>TQPALLRLSDHLLANYKKGVRPVRDWRKPTTVSIDVIMYAILNVDEKNQVLTTYIWYRQYWTDEFLQWTPEDFDNVTKLSIPTDSIWVPDILINEFVDVGKSPNIPYVYVHHRGEVQNYKPLQLVTACSLDIYNFPFDVQNCSLTFTSWLHTIQDINITLWRSPEEVRSDKSIFINQGEWELLEVFPQFKEFSIDISNSYAEMKFYVIIRRRPLFYAVSLLLPSIFLMVVDIVGFCLPPDSGERVSFKITLLLGYSVFLIIVSDTLPATAIGTPLIGVYFVVCMALLVISLAETIFIVRLV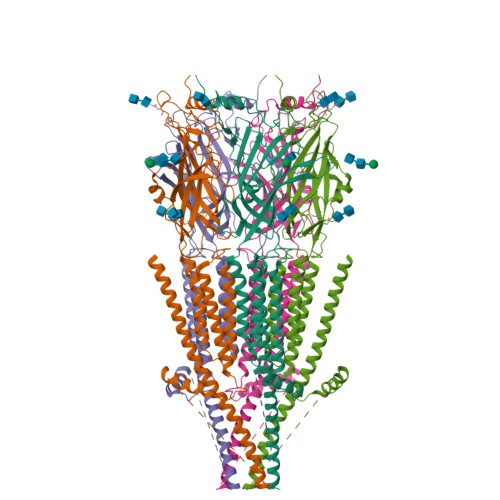HKQDLQRPVPDWLRHLVLDRIAWILCLGEQPMAHRPPATFQANKTDDCSGSDLLPAMGNHCSHVGGPQDLEKTPRGRGSPLPPPREASLAVRGLLQELSSIRHFLEKRDEMREVARDWLRVGYVLDRLLFRIYLLAVLAYSITLVTLWSIWHYS[5x]> YGSWEIDPKDLTFLKELGTGQFGVVKYGKWRGQYDVAIKMIKEGSMSEDEFIEEAKVMMNLSHEKLVQLYGVCTKQRPIFIITEYMANG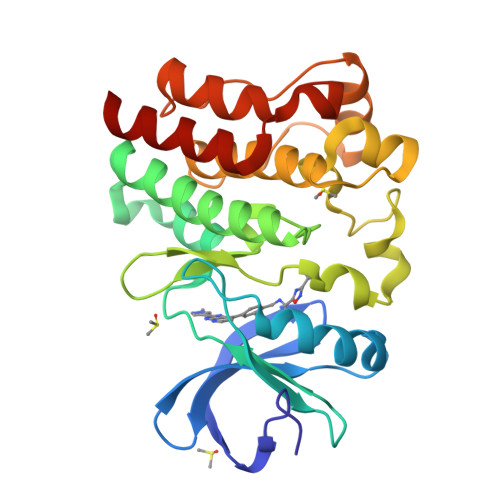CLLNYLREMRHRFQTQQLLEMCKDVCEAMEYLESKQFLHRDLAARNCLVNDQGVVKVSDFGLSRYVLDDEYTSSVGSKFPVRWSPPEVLMYSKFSSKSDIWAFGVLMWEIYSLGKMPYERFTNSETAEHIAQGLRLYRPHLASEKVYTIMYSCWHEKADERPTFKILLSNILDVMDEES>[8x]MSDSSPTINFINFNQTGTCISLGTSKGFKIFNCEPFGKFYSEDSGGYAIVEMLFSTSLLALVG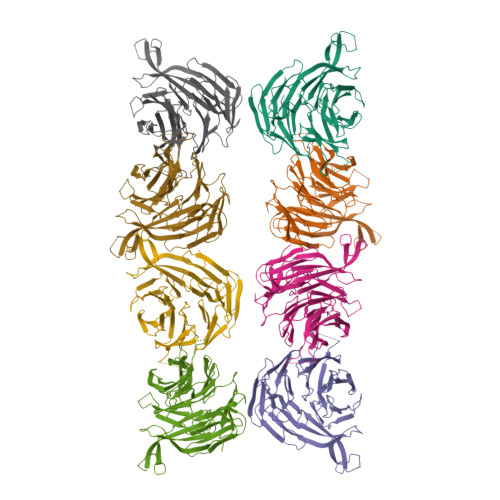IGDQPALSAARLRIINTKKHSIICEVTFPTSILSVKMNKSRLVVLLQEQIYIYDINTMRLLHTIETNPNPRGLMAMSPSVANSYLVYPSPPKVINSEIKAHATTNNITLSVGGNTETSFKRDQQDAGHSDISDLDQYSSFTKRDDADPTSSNGGNSSIIKNGDVIVFNLETLQPTMVIEAHKGEIAAMAISFDGTLMATASDKGTIIRVFDIETGDKIYQFRRGTYATRIYSISFSEDSQYLAVTGSSKTVHIFKLGHSMSNNKLDSDDSNMEEAAADDSSLDTTSIDALSDEENPTRLAREPYVDASRKTMGRMIRYSSQKLSRRAARTLGQIFPIKVTSLLESSRHFASLKLPVETNSHVMTISSIGSPIDIDTSEYPELFETGNSASTESYHEPVMKMVPIRVVSSDGYLYNFVMDPERGGDCLILSQYSILMD>[2x]MSGMKKLYEYTVTTLDEFLEKLKEFILNTSKDKIYKLTITNPKLIKDIGKAIAKAAEIADVDPKEIEEMIKAVEENELTKLVITIEQTDDKYVIKVELENEDGLVHSFEIYFKNKEEMEKFLELLEKLISKLSGS

pmcThe protein sequence design problem is to find, given a protein backbone structure of interest, an amino acid sequence that will fold to this structure. Here we describe a deep learning based protein sequence design method, ProteinMPNN, with outstanding performance in both in silico and experimental tests. We set out to develop a deep learning based protein sequence design method broadly applicable to design of monomers, cyclic oligomers, protein nanoparticles, and protein-protein interfaces.

We demonstrate the broad utility and high accuracy of ProteinMPNN using X-ray crystallography, cryoEM and functional studies by rescuing previously failed designs, made using Rosetta or AlphaFold, of protein monomers, cyclic homo-oligomers, tetrahedral nanoparticles, and target binding proteins. Incorporation of noise during training improves sequence recovery on protein structure models, and produces sequences which more robustly encode their structures as assessed using structure prediction algorithms. In contrast, sequences encoded by noised ProteinMPNN models are more accurately decoded into 3D coordinates by AlphaFold, likely because noised models focus more on overall topological features than fine local structural details (which are blurred during noising). In protein design calculations, the models trained with larger amounts of noise have the advantage of generating sequences which more strongly map to the target structures by prediction methods (this increases frequency of designs passing prediction based filters, and may correspondingly also increase the frequency of actual folding to the desired target structure). ProteinMPNN solves sequence design problems in a small fraction of the time (1.2 sec vs 258.8 sec on a single CPU for a 100 residue protein) required for physically based approaches such as Rosetta, which carry out large scale sidechain packing calculations, achieves much higher protein sequence recovery on native backbones (52.4% vs 32.9%), and most importantly, rescues previously failed designs made using Rosetta or AlphaFold for protein monomers, assemblies, and protein-protein interfaces. As illustrated in the accompanying paper (Wicky et al.), ProteinMPNN designs also have a much higher propensity to crystallize, greatly facilitating structure determination of designed proteins.2-(5-isothiocyanato-1-benzofuran-2-yl)-4,5-dihydro-1H-imidazole 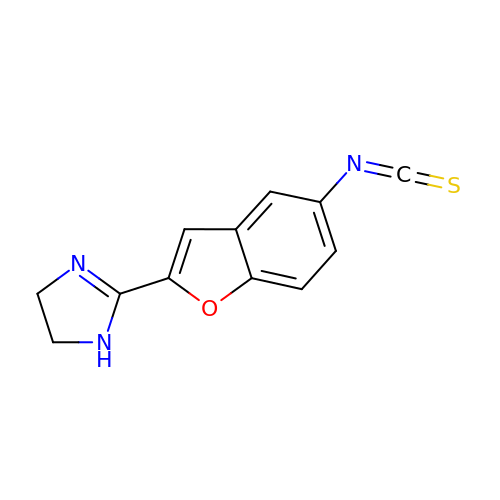| C12 H9 N3 O S | RUDBUHTXVGVWTA-UHFFFAOYSA-N> AKFEDKVDLYDDRGNLVEEQVPLEALSPLRNPAIKSIVQGIKRTVAVNLEGIENALKTAKVGGPACKIMGRELDLDIVGNAESIAAAAKEMIQVTEDDDTNVELLGGGKRALVQVPSARFDVAAEYSAAPLVTATAFVQAIINEFDVSMYDANMVKAAVLGRYPQSVEYMGANIATMLDIPQKLEGPGYALRNIMVNHVVAATLKNTLQAAALSTILEQTAMFEMGDAVGAFERMHLLGLAYQGMNADNLVFDLVKANGKEGTVGSVIADLVERALEDGVIKVEKELTDYKVYGTDDLAMWNAYAAAGLMAATM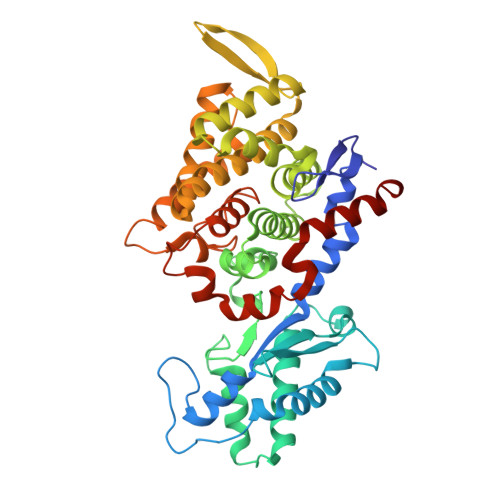VNQGAARAAQGVSSTLLYYNDLIEFETGLPSVDFGKVEGTAVGFSFFSHSIYGGGGPGIFNGNHIVTRHSKGFAIPCVAAAMALDAGTQMFSPEATSGLIKEVFSQVDEFREPLKYVVEAAAEIKNEI>MAHHHHHHMQDEMYMARALKLAARGRFTTHPNPNVGCVIVKDGEIVGEGFHYRAGEPHAEVHALRMAGDKAKGATAYVTLEPCSHHGRTPPCCDALIAAGVARVVAAMQDPNPQVAGRGLYRLQQAGIDVSHGLMMNEAEALNKGFLKRMRTGFPWIQLKMGASLDGRTAMASGESQWITSPQARRDVQRLRAQSHAILTSSATVLADDPALTVRWQELSADTQALYPQENLRQPLRIVIDSQNRVTPEHRIIQQQ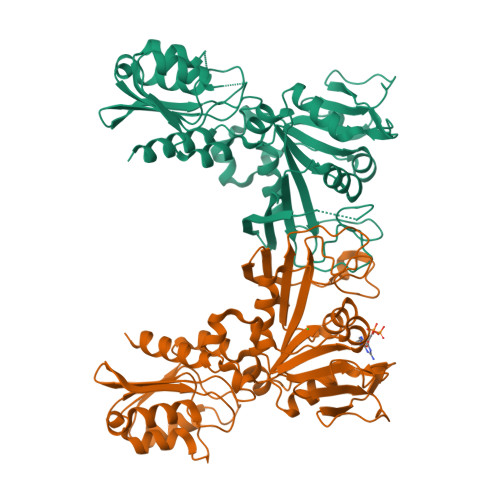GETLFARTHADERAWPDNVRTLLVPEHNGHLDLVLLMMQLGKQQVNSIWVEAGPTLAGALLQAGLVDELIVYIAPKLLGSDARGLCALPGLEKLSQAPHFKFNEIRQVGPDVCLHLTTA[2x]SARS‐CoV‐2 and SARS‐CoV share an otherwise non‐conserved part of non‐structural protein 3 (Nsp3), therefore named as “SARS‐unique domain” (SUD). Paip1 acts as a positive translation stimulator to regulate the key translation factor PABP in the host translation system. The three‐dimensional structure of the N‐terminal domain of SARS‐CoV SUD (“macrodomain II”, Mac2) in complex with the middle domain of Paip1, determined by X‐ray crystallography and small‐angle X‐ray scattering, provides insights into the structural determinants of the complex formation. In addition to receptor usage, the potential of a zoonotic virus to establish itself in a new host will depend on its ability to cope with the innate immune system of this host and possibly with its capability to use the host's protein synthesis machinery for its own benefit. Our study provides new insight on the latter aspect for SARS‐CoV by demonstrating that the SUD‐N (Mac2) domain interacts with the host cell translation apparatus via Paip1 and increases viral translation.

After trying many optimization methods and testing over 240 crystals at the synchrotron, we managed to collect a 3.5‐Å dataset. The structure of the Mac2:Paip1M complex was finally determined by first using the SAD data to position Mac2 in the asymmetric unit and then employing molecular replacement to locate Paip1M. One Mac2:Paip1M heterodimer exists per asymmetric unit. Mac2 adopts the typical α/β/α macrodomain fold. The main structural difference between the two Mac2 structures is located within the N‐terminal segment Lys389–Thr408. However, the β‐strand is replaced by a loop in the Mac2:Paip1M complex. In the Mac2:Paip1M complex, this region is a long loop, while it forms a β‐hairpin in free Paip1M. About 840 Å2 of the surface of Mac2 and 779 Å2 of the surface of Paip1M are buried upon complex formation, according to the PDBePISA server (complex formation significance score: 0.86 on a scale from 0 to 1, Krissinel & Henrick, 2007). The predominant interaction regions between Mac2 and Paip1M are confined to the N‐terminal loop Ile394–Leu407 of Mac2 and to α5 (Arg160–Arg168), the central loop (Ile204–Thr212), and the N‐terminal half of α7 (Ala214–Glu223) of Paip1M. Taken together, the N‐terminal Lys389–Thr404 region of Mac2 is indispensable for the interaction with Paip1M.

> GSHMKIKACIDEVTTTLEETKFLTNKLLLFADINGKLYHDSQNMLRGEDMSFLEKDAPYMVGDVITSGDITCVVIPSKKAGGTTEMLSRALKKVPVDEYITTYPGQGCAGYTLEEAKTALKKCKSAFYVLPSEAPNAKEEIL;> GSHMASMTGGQQMGRGSTLSEYVQDFLNHLTEQPGSFETEIEQFAETLNGCVTTDDALQELVELIYQQATSIPNFSYMGARLCNYLSHHLTISPQSGNFRQLLLQRCRTEYEVKDQAAKGDEVTRKRFHAFVLFLGELYLNLEIKGTNGQVTRADILQVGLRELLNALFSNPMDDNLICAVKLLKLTGSVLEDAWKEKGKMDMEEIIQRIENVVLDANCSRDVKQMLLKLVELRSS>GQIQISKHVKDVGLPSIHTPTKTKLQPSVFYDIFPGSKEPAVLTEKDPRLKVDFDSALFSKYKGNTECSLNEHIQVAVAHYSAQLATLDIDPQPIAMEDSVFGMDGLEALDLNTSAGYPYVTLGIKKKDLINNKTKDISKLKLALDKYDVDLPMITFLKDELRKKDKIAAGKTRVIEASSINDTILFRTVYGNLFSKFHLNPGVVTGCAVGCDPETFWSKIPLMLDGDCIMAFDYTNYDGSIHPIWFKALGMVLDNLSFNPTLINRLCNSKHIFKSTYYEVEGGVPSGCSGTSIFNSMINNIIIRTLVLDAYKHIDLDKLKII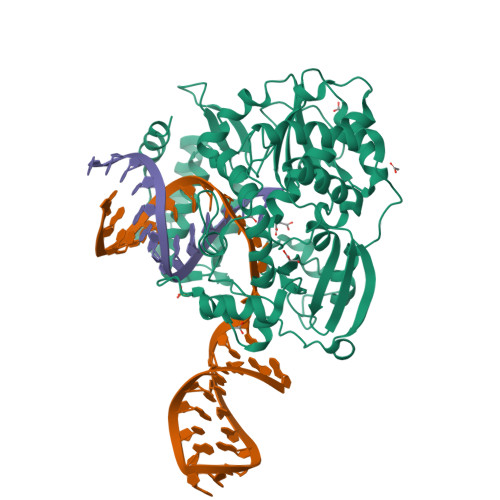AYGDDVIFSYKYKLDMEAIAKEGQKYGLTITPADKSSEFKELDYGNVTFLKRGFRQDDKYKFLIHPTFPVEEIYESIRWTKKPSQMQEHVLSLCHLMWHNGPEIYKDFETKIRSVSAGRALYIPPYELLRHEWYEKF[4x]>SSDTTPCCFAYIARPLPRAHIKEY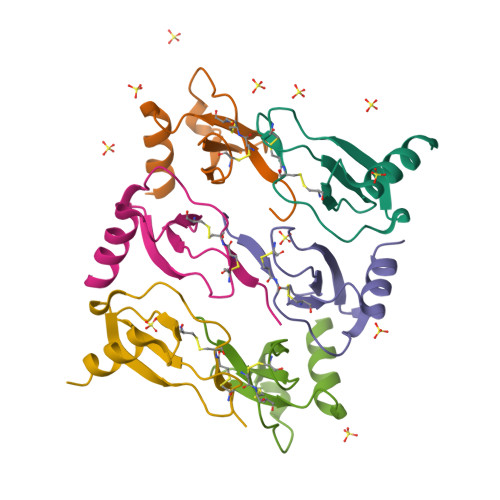FYTSGKCSNPAVVFVTRKNRQVCANPEKKWVREYINSLEMS[6x]methyl 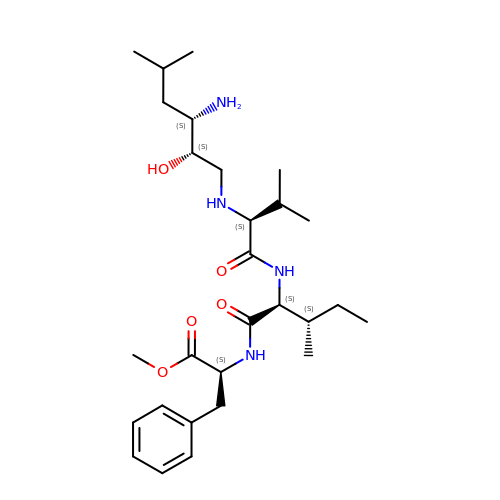N-[(2S,3S)-3-amino-2-hydroxy-5-methylhexyl]-L-valyl-L-isoleucyl-L-phenylalaninate | C28 H48 N4 O5 | JAELWYBMQVXTOC-ACUVNOOJSA-N> MGSHQERPLIGLLFSETGVTADIERSQRYGALLAVEQLNREGGVGGRPIETLSQDPGGDPDRYRLCAEDFIRNRGVRFLVGCYMSHTRKAVMPVVERADALLCYPTPYEGFEYSPNIVYGGPAPNQNSAPLAAYLIRHYGERVVFIGSDYIYPRESNHVMRHLYRQHGGTVLEEIYIPLYPSDDDLQRAVERIYQARADVVFSTVVGTGTAELYRAIARRYGDGRRPPIASLTTSEAEVAKMESDVAEGQVVVAPYFSSIDTPASRAFVQACHGFFPENATITAWAEAAYWQTLLLGRAAQAAGNWRVEDVQRHLYDIDIDAPQGPVRVERQNNHSRLSSRIAEIDARGVFQVRWQSPEPIRPDPYVVVHNLDDWSASMG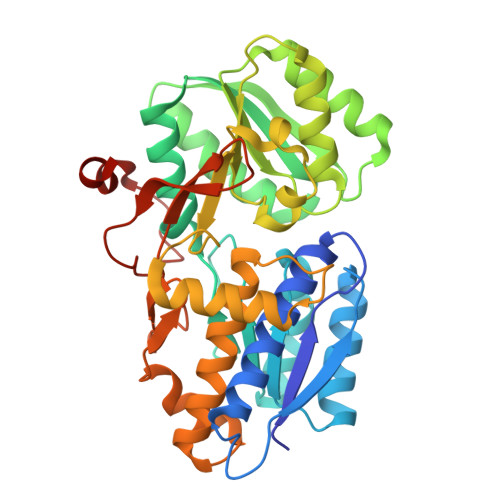GGPLP> MSDI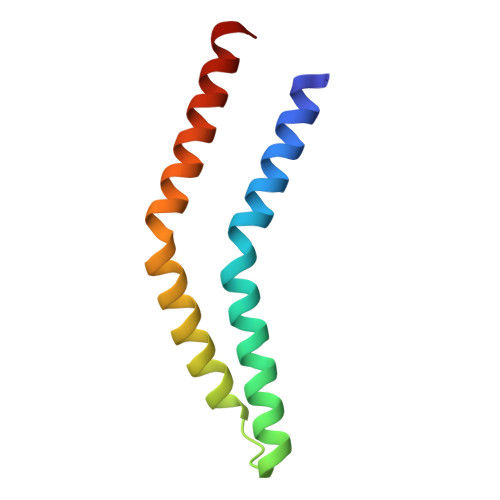VYMGNKALYLILIFSLWPVGIATVIGLSIGLLQTVTQLQEQTLPFGIKLIGVSISLLLLSGWYGEVLLSFCHEIMFLIKSGV~{N}-[3-(azepan-1-ylsulfonyl)-4-methyl-phenyl]-2-[4,4-dimethyl-2,5-bis(oxidanylidene)imidazolidin-1-yl]ethanamide | C20 H28 N4 O5 S | 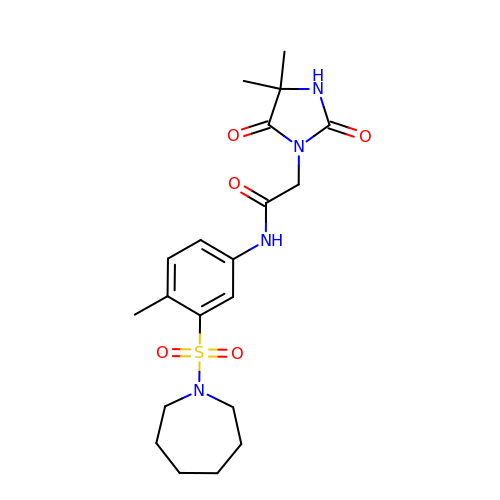ZHCSIBLDPZYQBH-UHFFFAOYSA-N>GAMSHPHDSKVFPDLPEHQDNPSQLRLQHDGLATDDKARLEPM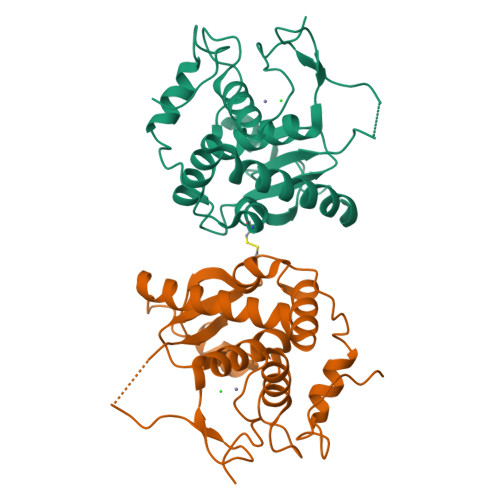CLAEYLISGPGGMDPDIEIDDDTYDECREVLSRILEDAYTQSGTFRRLMNYAYDQELHDVEQRWLLGAGENFGTTVTDEDLESSEGRKVIALNLDDTDDDSIPEYYESNDGPQQFDTTRSFIHQVVHALTHLQDKEDSNPRGPVVEYTNIILKEMGHTSPPRIAYEFSN[2x]>ESLQRKRLCKARLYDVTRHHVKHKRLKPLIEHIDEYCNEKDENKGDVLFFLLRSHLYDTGNRSMAEQIDTLWHGESLSCMTPEECLGMRLDMLMTKNQYSKEYNILKERGFSTLCPPKQLDAIEKTLMPGTARYSIEGMDYSEHYFHSPVKMTGDLEVHSGETLEPDSVTMDFHEYVPDFPCPNTKGVRFPYAHAVAKTLEELEDEIVNGLKKLGRDPNDPTLVIHTICKDGADGMGDVSVHKEKSDHLLPDKALRFSFCVLRCSVMHKDTEVTIYEDPNPNSVRSNRPVLECIGDENDDGTVAVCVGPIECQRLLMKDKIMRVHMSDGTQRAHYLTFFNSMVDEKWDRAHGGLAGAGSKYLCTLCEAVRDEALEKAGSYKITRTLKKI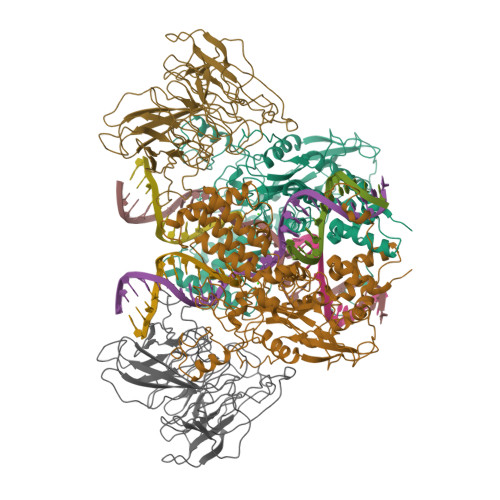EVTASKMKYESQEKDTFGVKGYPLLTTEPWERGIDATHTDINMGNYFKSLIVREMAQVHSWAKTANVKKQIVDAESKLDKHLKESLGLNPTLMMAGNYARELFKAEHADKLVALVDKPDRKSALVEVLAKFRQLRKVYRANWPLNDMSDEVRQYKAKAVEMANDLKTHFPYAPCTNYLHKVIEHVQELIEHPSGVGSVGALSSEGNEAGNKLFRQLRLGHARKGNTYNGLRDVLCTHWLYTSKTLRDKAAXXXXXXXXXXXXXXXXXXX[2x];>MSSGPIFSSLVTDSSRSSRKKSDSALGTEFTVVCDRVPLRDPSPTVQRFLCFVFDNGSGAMSTLPIDVGGEGISLSDMKEVKAMPHIASGCTAVWGPPLPPKPGKDTKQVILWGGLDKRRWCCSNDLTQVDITITPKTTTAKVSILPADKQDGVPSPRTGHTLVAISSLQAILFGGLELASRHARLGTCAQSCKDGYFYLLDMTTLRWNKLPLPPLVPRAYHSSTWVPASSTMVIVGGITYSGHCPSERLSVSDVVCLKISDTSQYTLTEIHMEGVRDSYVSSSSASALCDDRFVLYGGYHHDKSGLHPPEPSRDLYVMNLQTKKAVVHHAPTRMASAGHTCLRLIDNSVVMIGGTCKSVNCCTNL[2x]(2~{S},3~{S},4~{R},5~{S},6~{R})-2-(fluoranylmethyl)-6-[(2~{R},3~{R},4~{S},5~{S},6~{S})-6-(fluoranylmethyl)-3,4,5-tris(oxidanyl)oxan-2-yl]oxy-oxane-3,4,5-triol 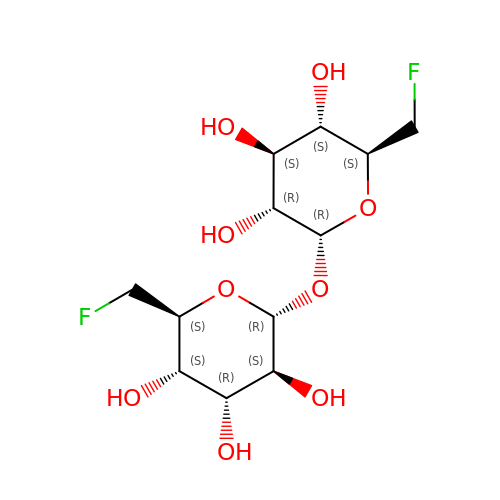| C12 H20 F2 O9 | CZAGHLGJQHEHTN-YDHPHUQESA-N> GASAKEKFTSLSPAEFFKRNPELAGFPNPARALYQTVRELIENSLDATDVHGILPNIKITIDLIDDARQIYKVNVVDNGIGIPPQEVPNAFGRVLYSSKYVNRQTRGMYGLGVKAAVLYSQMHQDKPIEIETSPVNSKRIYTFKLKIDINKNEPIIVERGSVENTRGF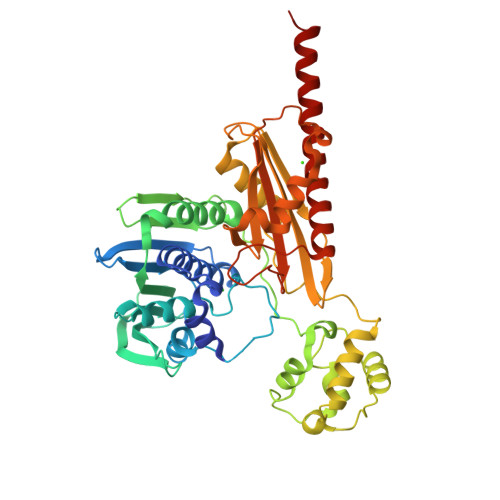HGTSVAISIPGDWPKAKSRIYEYIKRTYIITPYAEFIFKDPEGNVTYYPRLTNKIPKPPQEVKPHPYGVDREEIKILINNLKRDYTIKEFLVNEFQSIGDTTADKILELAGLKPNKKVKNLTEEEITRLVETFKKYEDFRSPSADSLSVIGEDLIELGLKKIFNPDFAASITRKPKAYQGHPFIVEAGVAFGGSIPVGEEPIVLRYANKIPLIYDEKSDVIWKVVEELDWKRYGIESDQYQMVVMVHLCSTKIPYKSAGKESIAEVEDIEKEIKNALMEVARKLKQYLSEKRKEQEAKKKLLA>IQTTAPPVKESSFVEKMKKTGRNIIVFYGSQTGTAEEFANRLSKDAHRYGMRGMSADPEEYDLADLSSLPEIDKSLVVFCMATYGEGDPTDNAQDFYDWLQETDVDLTGVKFAVFGLGNKTYEHFNAMGKYVDQRLEQLGAQRIFELGLGDDDGNLEEDFITWREQFWPAVCEFFGVEATGEESSIRQYELVVHEDMDVAKVYTGEMGRLKSYENQKPPFDAKNPFLAAVTANRKLNQGTERHLMHLELDISDSKIRYESGDHVAVYPANDSALVNQIGEILGADLDVIMSLNNLDEESNKKHPFPCPTTYRTALTYYLDITNPPRTNVLYELAQYASEPSEQEHLHKMASSSGEGKELYLSWVVEARRHILAILQDYPSLRPPIDHLCELLPRLQARYYSIASSSKVHPNSVHICAVAVEYEAKSGRVNKGVATSWLRAKEPAGENGGRALVPMFVRKSQFRLPFKSTTPVIMVGPGTGIAPFMGFIQERAWLREQGKEVGETLLYYGCRRSDEDYLYREELARFHKDGALTQLNVAFSREQAHKVYVQHLLKRDREHLWKLIHEGGAHIYVCGDARNMAKDVQNTFYDIVAEFGP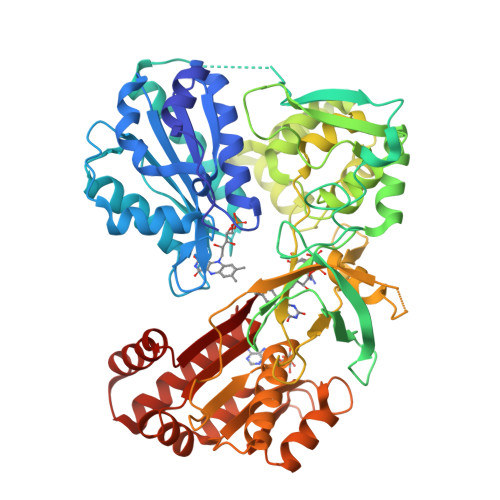MEHTQAVDYVKKLMTKGRYSLDVWS[2x]> AGYDKDLVEALERDIVSRNPSIHWDDIADLEEAKKLLREAVVLPMWMPDFFKGIR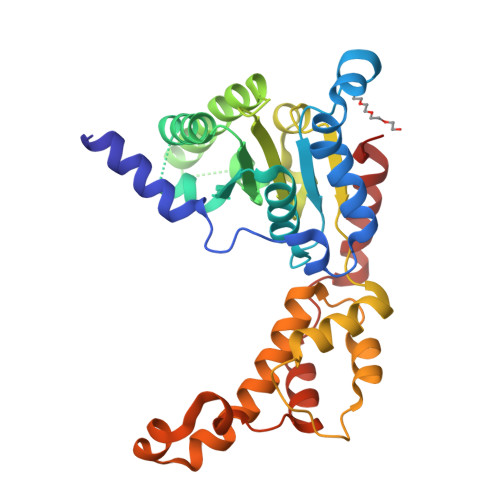RPWKGVLMVGPPGTGKTMLAKAVATECGTTFFNVSSSTLTSKYRGESEKLVRLLFEMARFYAPTTIFIDQIDSICSRRGTSDEHEASRRVKSELLIQMDGVGGALENDDPSKMVMVLAATNFPWDIDEALRRRLEKRIYIPLPTAKGRAELLKINLREVELDPDIQLEDIAEKIEGYSGADITNVCRDASLMAMRRRINGLSPEEIRALSKEELQMPVTKGDFELALKKIAKSVSAADLEKYEKWMVEFGSA>[2x]SYDKVSQAKSIIIGTKQTVKALKRGSVKEVV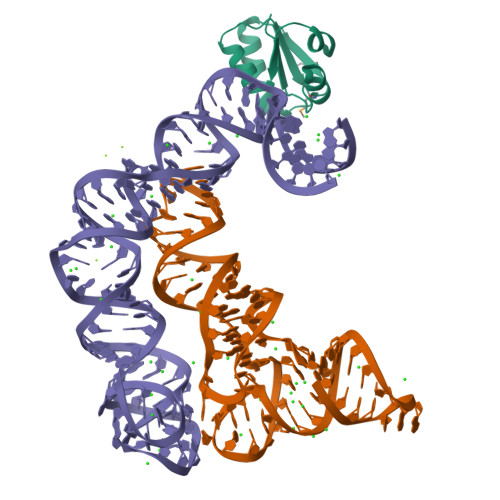VAKDADPILTSSVVSLAEDQGISVSMVESMKKLGKACGIEVGAAAVAIIL>MASQSSVAVISSAAARGESFPDSKKPIGSVRFQQPLRLSFSYCKSGNMSSRICAMAKPNDAETLSSSV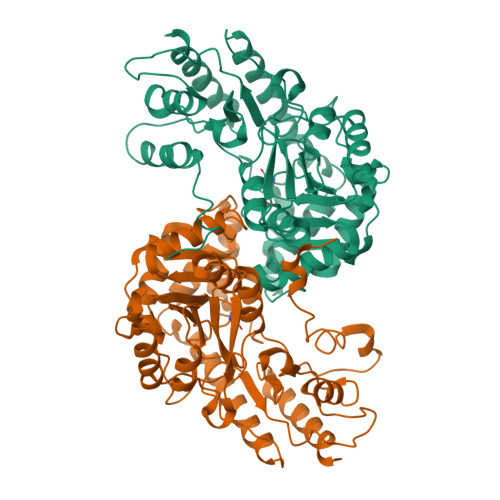DMSLSPRVQSLKPSKTMVITDLAATLVQSGVPVIRLAAGEPDFDTPKVVAEAGINAIREGFTRYTLNAGITELREAICRKLKEENGLSYAPDQILVSNGAKQSLLQAVLAVCSPGDEVIIPAPYWVSYTEQARLADATPVVIPTKISNNFLLDPKDLESKLTEKSRLLILCSPSNPTGSVYPKSLLEEIARIIAKHPRLLVLSDEIYEHIIYAPATHTSFASLPDMYERTLTVNGFSKAFAMTGWRLGYLAGPKHIVAACSKLQGQVSSGASSIAQKAGVAALGLGKAGGETVAEMVKAYRERRDFLVKSLGDIKGVKISEPQGAFYLFIDFSAYYGSEAEGFGLINDSSSLALYFLDKFQVAMVPGDAFGDDSCIRISYATSLDVLQAAVEKIRKALEPLRATVSV[6x]> AIGEFMVSLPRMVYPQPKVLTPCRKDVLVVTPWLAPIVWEGTFNIDILNEQFRLQNTTIGLTVFAIKKYVAFLKLFLETAEKHFMVGHRVHYYVFTDQPAAVPRVTLGTGRQLSVLEVGAYKRWQDVSMRRMEMISDFCERRFLSEVDYLVCVDVDTEFRDHVGVEILTPLFGTLHPSFYGSSREAFTYERRPQSQAYIPKDEG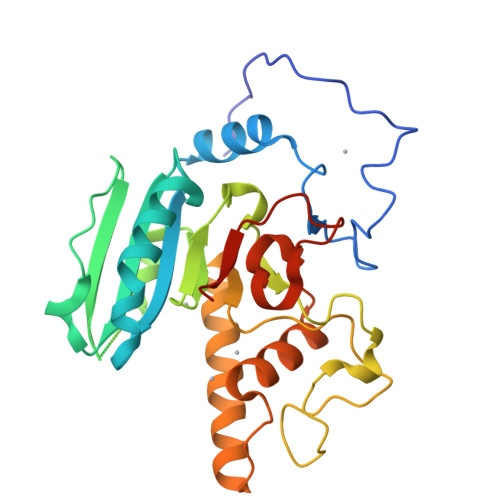DFYYMGAFFGGSVQEVQRLTRACHQAMMVDQANGIEAVWHDESHLNKYLLRHKPTKVLSPEYLWDQQLLGWPAVLRKLRFTAVPKNHQAVRNP> MASEKSLEEKQAENTFGWAAMDSSGVLSPFTFSRRATGEEDVRLKVLYCGICHSDLGCIKNEWGWCSYPLVPGHEIVGIATEVGSKVTKFKVGDRVGVGCMVGSCGTCQNCTQNQESYCPEVIMTCASAYPDGTPTYGGFSNQMVANEKFVIRIPNSLPLDAAAPLLCAGSTVYSAMKFYGLCSQGLHLGVVGLGGL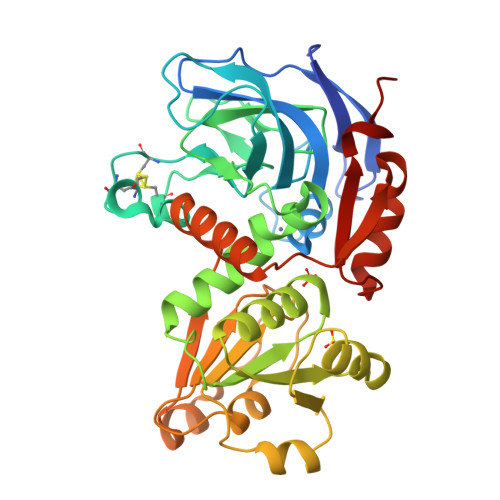GHVAVKFAKAFGMKVTVISTSLGKKEEAINQLGADSFLINTDTEQMQGAMEVMDGIIDTVSALHPIEPLLGLLKSHQGKLIIVGLPNKQPELPVFSLINGRKMIGGSAVGGVKETQEMIDFAAEHNITADIEIVPMDYVNTAMERLEKGDVKFRFVIDVENTLVAAQT> SRTNIDIDDELAAEVMRRFGLTTKRAAVDLALRR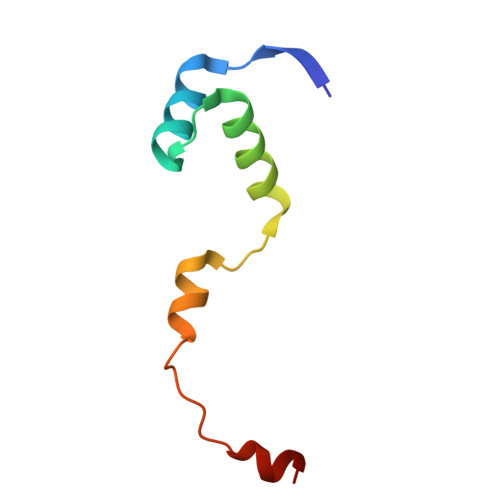LVGSPLSREFLLGLEGVGWEGDLDDLRS> MPVKRSLKLDGLLEENSFDPSKITRKKSVITYSPTTGTCQMSLFASPTSSEEQKHRNGLSNEKRKKLNHPSLTESKESTTKDNDEFMMLLSKVEKLSEEIMEIMQNLSSIQALEGSRELENLIGISCASHFLKREMQ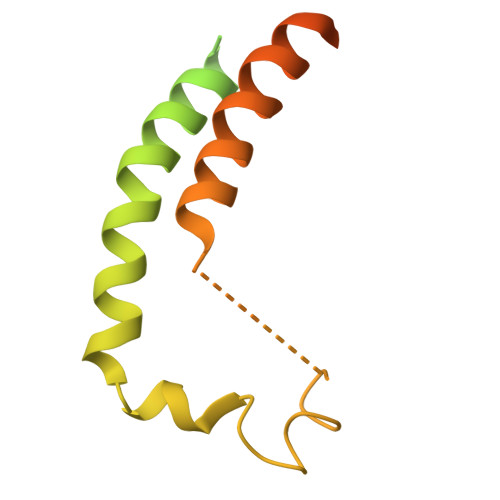KTKELMTKVNKQKLFEKSTGLPHKASRHLDSYEFLKAILN>LNSINTNPGALLALQNLNSTNTELAATQGRINTGKKVANAKDNGAIWSMAKMQSATASSLNSVKDSLQRGQSTIDVALAAGDTITDL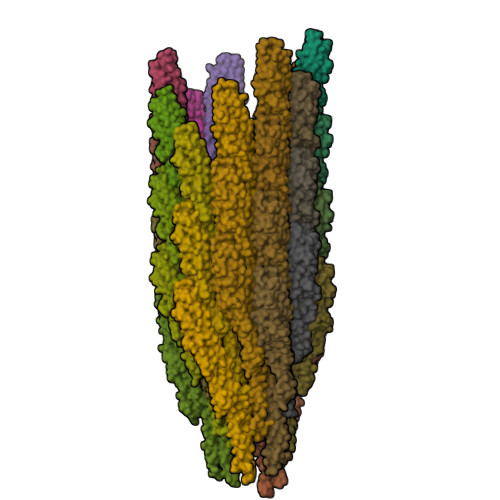LTKMKEKALAASDTSLNTASFNALKADFESLRDQLQKAATNAKFNGVSLADGSTTKLSFLANEDGSNFTVTAQTLSLTGIGLTATSTFTDAATAKTMIATITTSLQTATNKLSSLGTSSVGLDTHLTFVGKLQDSLDAGVGNLVDADLAKESAKLQSLQTKQQLGVQALSIANQTPQTILSLF[37x]> MPAIMTMLADHAARQLLDFSQKLDINLLDNVVNCLYHGEGAQQRMAQEVLTHLKEHPDAWTRVDTILEFSQNMNTKYYGLQILENVIKTRWKILPRNQCEGIKKYVVGLIIKTSSDPTCVEKEKVYIGKLNMILVQILKQEWPKHWPTFISDIVGASRTSESLCQNNMVILKLLSEEVFDFSSGQITQVKSKHLKDSMCNEFSQIFQLCQFVMENSQNAPLVHATLETLLRFLNWIPLGYIFETKLISTLIYKFLNVPMFRNVSLKCLTEIAGVSVSQYEEQFVTLFTLTMMQLKQMLPLNTNIRLAYSNGKDDEQNFIQNLSLFLCTFLKEHDQLIEKRLNLRETLMEALHYMLLVSEVEETEIFKICLEYWNHLAAELYRESPFSTSASPLLSGSQHFDVPPRRQLYLPMLFKVRLLMVSRMAKPEEVLVVENDQGEVVREFMKDTDSINLYKNMRETLVYLTHLDYVDTERIMTEKLHNQVNGTEWSWK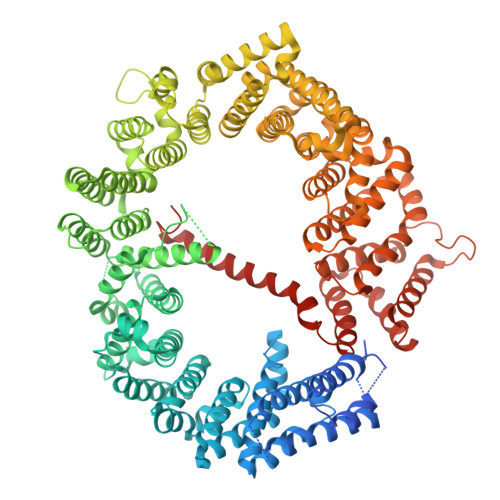NLNTLCWAIGSISGAMHEEDEKRFLVTVIKDLLGLCEQKRGKDNKAIIASNIMYIVGQYPRFLRAHWKFLKTVVNKLFEFMHETHDGVQDMACDTFIKIAQKCRRHFVQVQVGEVMPFIDEILNNINTIICDLQPQQVHTFYEAVGYMIGAQTDQTVQEHLIEKYMLLPNQVWDSIIQQATKNVDILKDPETVKQLGSILKTNVRACKAVGHPFVIQLGRIYLDMLNVYKCLSENISAAIQANGEMVTKQPLIRSMRTVKRETLKLISGWVSRSNDPQMVAENFVPPLLDAVLIDYQRNVPAAREPEVLSTMAIIVNKLGGHITAEIPQIFDAVFECTLNMINKDFEEYPEHRTNFFLLLQAVNSHCFPAFLAIPPTQFKLVLDSIIWAFKHTMRNVADTGLQILFTLLQNVAQEEAAAQSFYQTYFCDILQHIFSVVTDTSHTAGLTMHASILAYMFNLVEEGKISTSLNPGNPVNNQIFLQEYVANLLKSAFPHLQDAQVKLFVTGLFSLNQDIPAFKEHLRDFLVQIKEFAGEDTSDLFLEEREIALRQADEEKHKRQMSVPGIFNPHEIPEEMCD> MATPSFGNSSPQLTFTHVANFMNDAAADVSAVDAKQLAQIRQFLKANKTNLIESLNTIRQNVTSSGDHNKLRSTIANLLQINVDNDPFFAQSEDLSHAVEFFMSERSSRLHIVYSLLVNPDIDLETYSFIDNDRFNVVGKLISIISSVIQNYDIITASSLAHDYNNDQDMFTIVSLVQLKKFSDLKFILQILQILNLMILNTKVPVDIVNQWFLQYQNQFVEFCRNINSTDKSIDTSSLQLYKFQNFQDLSYLSETLISRISSLFTITTILILGLNTSIAQFDIQSPLYMDTETFDTVNSALENDVATNIVNEDPIFHPMIHYSWSFILYYRRALQSSESFDDSDITKFALFAESHDVLQKLNTLSEILSFDPVYTTVITVFLEFSLNFIPITASTSRVFAKIISKAPEQFIENFLTNDTFEKKLSIIKAKLPLLNESLIPLINLALIDTEFANFELKDICSFAVTKSSLNDLDYDLIADTITNSSSSSDIIVPDLIELKSDLLVAPPLENENSNCLLSIPKSTKGKILTIKQQQQQQQQQNGQQPPTTSNLIIFLYKFNGWSLVGRILQNLLHSYMEKGTQLDDLQHELMISIIKLVTNVVDPKTSIEKSSEILSYLSNSLDTSASTINGASIIQVIFEIFEISLQRKDYTSIVQCCEFMTMLTPNYLHLVSSYLNKSDLLDKYGKTGLSNMILGSVELSTGDYTFTIQLLKLTKVFIRESLSLKNIHISKRSKIDIINKLILHAIHIFESYYNWKYNNFLQKFEIAFHLTLIFYDVLHDVFTINPHQKDQLIISSSANKLLQLFLTPMDSIDLAPNTLTNILISPLNTTTKILGDKILGNLYSKVMNNSFKLCTLLIAIRGSNRDLKPSNLEKLLFINSSKLVDVYTLPSYVHFKVQIIELLSYLVEAPWNDDYPFLLSFLGEAKSMAFLKEVLSDLSSPVQDWNLLRSLYIFFTTLLESKQDGLSILFLTGQFASNKKINDESSIDKKSSILTVLQKNSLLLDSTPEEVSCKLLETITYVLNTWTNSKIFIKDPKFVNSLLAKLKDSKKLFQKKENLTRDETVSLIKKYKLISRIVEIFALCIYNSTDSNSEILNFLNQEDLFELVHHFFQIDGFNKTFHDELNLKFKEKWPSLELQSFQKIPLSRINENENFGYDIPLLDIVLKADRSWNEPSKSQTNFKEEITDASLNLQYVNYEISTAKAWGALITTFVKRSTVPLNDGFVDLVEHFLKLNIDFGSDKQMFTQIYLERIELSFYILYSFKLSGKLLKEEKIIELMNKIFTIFKSGEIDFIKNIGKSLKNNFYRPLLRSVLVLLELVSSGDRFIELISDQLLEFFELVFSKGVYLILSEILCQINKCSTRGLSTDHTTQIVNLEDNTQDLLLLLSLFKKITNVNPSKNFNVILASSLNEVGTLKVILNLYSSAHLIRINDEPILGQITLTFISELCSIEPIAAKLINSGLYSVLLESPLSVAIQQGDIKPEFSPRLHNIWSNGLLSIVLLLLSQFGIKVLPETCLFVSYFGKQIKSTIYNWGDNKLAVSSSLIKETNQLVLLQKMLNLLNYQELFIQPKNSDDQQEAVELVIGLDSEHDKKRLSAALSKFLTHPKYLNSRIIPTTLEEQQQLEDESSRLEFVKGISRDIKALQDSLFKDV

Nuclear pore complexes (NPCs), embedded in NE, are the massive bidirectional transport channels between the nucleus and the cytoplasm. The NPC is the largest proteinaceous assembly in vivo, which consists of ~550–1000 molecules of ~30 different nucleoporins (Nups) with the molecular mass of 60–120 MDa from yeast to human, and are the sole gatekeepers controlling the nucleocytoplasmic transport of macromolecules. As the core scaffold of the NPC, the inner ring (IR) attaches itself to the cytoplasmic, nucleoplasmic and luminal rings (CR, NR and LR), and is directly involved in the formation of the central transport channel of the NPC. In summary, our cryo-EM structures describe in detail the hierarchical assembly of the scNPC IR, which consists of 192 molecules of 8 Nups with an 8-fold rotational symmetry.

Nup188 and Nup192, two of the largest subunits in the NPC, are evolutionary conserved homologous nucleoporins. Since the density maps of Nup188 and Nup192 are not completely resolved in the IR monomer map, we next performed SPA of the purified Nup188 and Nup192 samples, respectively, and successfully obtained the full-length structure of Nup188 at a resolution of 2.81 Å. Overall Nup188 appears to be a cray shape with a dimension of ∼170 × 90 × 65 Å. The Neck domain is at the corner followed by a crescent C-terminal domain (CTD). The clamp, Neck and CTD domains further form a large right-handed super-helical ring that resembles the letter “S” comprising 52 stacked helices. Surrounding the axis of the “S”, two layers of concentric α-helices spiral up in parallel and are referred to as the outer/inner layer with respect to their distances to the axis, which probably enables Nup188, like a spring, to stretch and shrink to a certain extent. The relatively poor density of the SH3-like domain and the tail of CTD represent intrinsic flexibility of these regions, which is consistent with their roles in mediating interactions with neighboring IR monomers. Moreover, the feature of Nup188 distinguishing it from Nup192 is the existence of the N-terminal SH3-like domain, which is composed of several β-strands and loops. The overall S-shaped conformation shared by Nup188 and Nup192 may play important roles in regulating and maintaining the malleability of IR.> GPGSDTERPVVNVPSEITVYRGESFEYFATVTDNSNAFDLAKTVVRWLYSNQPGRGTEWLQYSVTQVGNQLKVRIFGNVPIDTTIGDYTRYVVATDAAGNVN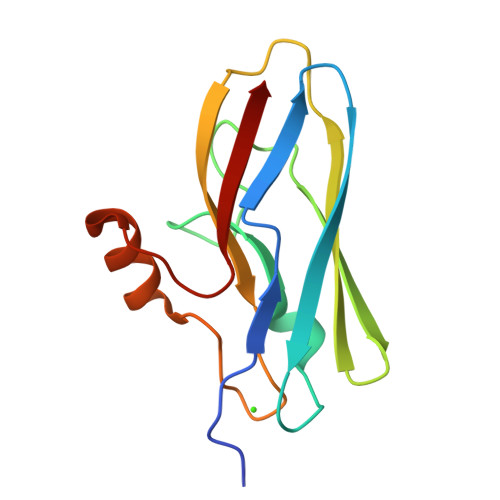ATQTEMGNAAVDKTSVNGQFKLIIR> TCGGCGCC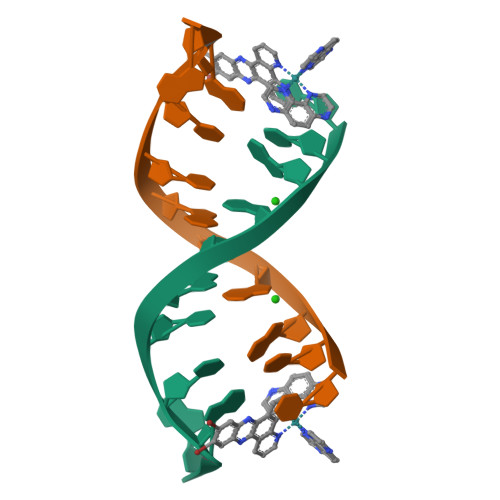GA> MHHHHHHHHMSSSDEQPRPRRRNQDRQHPNQNRPVLGRTERDRNRRQFGQNFLRDRKTIARIAETAELRPDLPVLEAGPGEGLLTRELADRARQVTSYEIDPRLAKSLREKLSGHPNIEVVNADFLTAEPPPEPFAFVGAIPYGITSAIVDWCLEAPTIETATMVTQLEFARKRTGDYGRWSRLTVMTWPLFEWEFVEKVDRRLFKPVPKVDSAIMRLRRRAEPLLEGAAL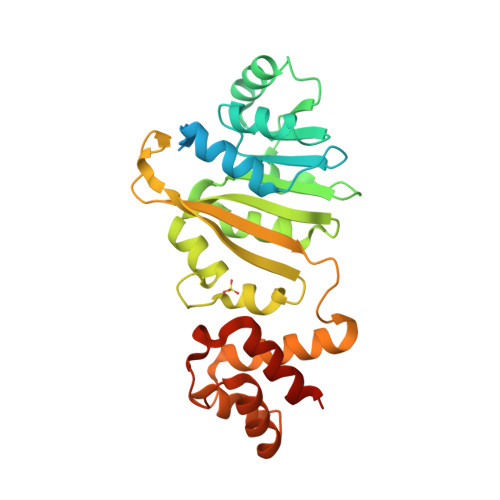ERYESMVELCFTGVGGNIQASLLRKYPRRRVEAALDHAGVGGGAVVAYVRPEQWLRLFERLDQKNEPRLE> GLSDELEEVIVEKTKQTLASVSSGPKHTQSVPALTANETGATLPTRPSDNVETRTTYMHFNGSETDVESFLGRAACVHVTEIKNKNAAGLDNHRKEGLFNDWKINLSSLVQLRKKLELFTYVRFDSEYTILATASQPEASSYSSNLTVQAMYVPPGAPNPKEWDDYTWQSASNPSVFFKVGETSRFSVPFVGIASAYNCFYDGYSHDDPDTPYGITVLNHMGSMAFRVVNEHDVHTTIVKIRVYHRAKHVEA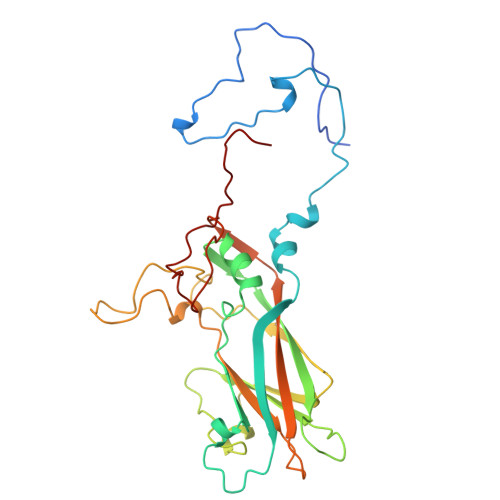WIPRAPRALPYVSIGRTNYPRDSKTIVKKRTNIKTY>[6x]SVRDELRWVF;>MPKALRFLGWPVLVG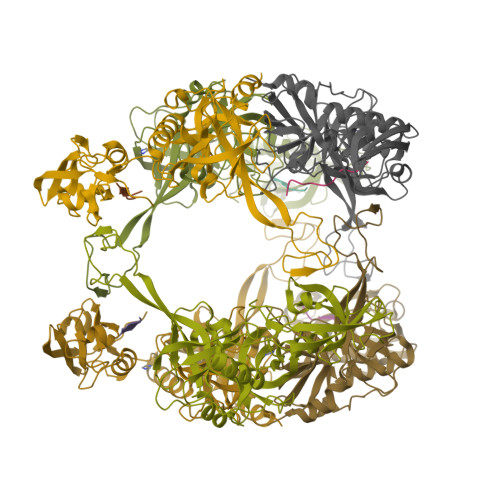VLLALLIIQHNPELVGLPRQEVHVEQAPLLSRLQEGPVSYANAVSRAAPAVANLYTTKMVSKPSHPLFDDPMFRRFFGDNLPQQKRMESSLGSAVIMSAEGYLLTNNHVTAGADQIIVALRDGRETIAQLVGSDPETDLAVLKIDLKNLPAMTLGRSDGIRTGDVCLAIGNPFGVGQTVTMGIISATGRNQLGLNTYEDFIQTDAAINPGNSGGALVDAAGNLIGINTAIFSKSGGSQGIGFAIPTKLALEVMQSIIEHGQVIRGWLGVEVKALTPELAESLGLGETAGIVVAGVYRDGPAARGGLLPGDVILTIDKQEASDGRRSMNQVARTRPGQKISIVVLRNGQKVNLTAEVGLRPPP[6x]>[2x]MGYTVAVVGATGAVGAQMIKMLEESTLPIDKIRYLASARSAGKSLKFKDQDITIEETTETAFEGVDIALFSAGSSTSAKYAPYAVKAGVVVVDNTSYFRQNPDVPLVVPEVNAHALDAHNGIIACPNCSTIQMMVALEPVRQKWGLDRIIVSTYQAVSGAGMGAILETQRELREVLNDGVKPCDLHA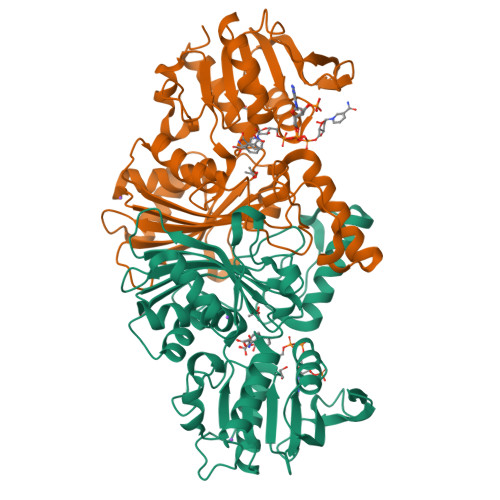EILPSGGDKKHYPIAFNALPQIDVFTDNDYTYEEMKMTKETKKIMEDDSIAVSATCVRIPVLSAHSESVYIETKEVAPIEEVKAAIAAFPGAVLEDDVAHQIYPQAINAVGSRDTFVGRIRKDLDAEKGIHMWVVSDNLLKGAAWNSVQIAETLHERGLVRPTAELKFELKLEHHHHHH>MSLFGTTSGFGTSGTSMFGSATTDNHNPMKDIEVTSSPDDSIGCLSFSPPTLPGNFLIAGSWANDVRCWEVQDSGQTIPKAQQMHTGPVLDVCWSDDGSKVFTASCDKTAKMWDLSSNQAIQIAQHDAPVKTIHWIKAPNYSCVMTGSWDKTLKFWDTRSSNPMMVLQLPERCYCADVIYPMAVVATAERGLIVYQLENQPSEFRRIESPLKHQHRCVAIFKDKQNKPTGFALGSIEGRVAIHYINPPNPAKDNFTFKCHRSNGTNTSAPQDIYAVNGIAFHPVHGTLATVGSDGRFSFWDKDARTKLKTSEQLDQPISAC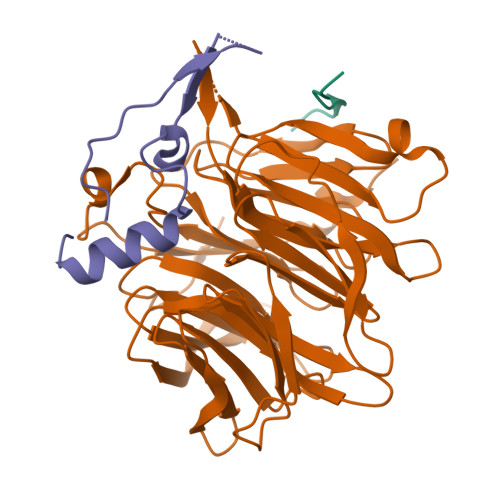CFNHNGNIFAYASSYDWSKGHEFYNPQKKNYIFLRNAAEELKPRNKK[2x];>MFNKSFGTPFGGGTGGFGTTSTFGQNTGFGTTSGGAFGTSAFGSSNNTGGLFGNSQTKPGGLFGTSSFSQPATSTSTGFGFGTSTGTANTLFGTASTGTSLFSSQNNAFAQNKPTGFGNFGTSTSSGGLFGTTNTTSNPFGSTSGSLFGPSSFTAAPTGTTIKFNPPTGTDTMVKAGVSTNISTKHQCITAMKEYESKSLEELRLEDYQANRKGPQNQVGAGTTTGLFGSSPATSSATGLFSSSTTNSGFAYGQNKTAFGTSTTGFGTNPGGLFGQQNQQTTSLFSKPFGQATTTQNTGFSFGNTSTIGQPSTNTMGLFGVTQASQPGGLFGTATNTSTGTAFGTGTGLFGQTNTGFGAVGSTLFGNNKLTTFGSSTTSAPSFGTTSGGLFGNKPTLTLGTNTNTSNFGFGTNTSGNSIFGSKPAPGTLGTGLGAGFGTALGAGQASLFGNNQPKIGGPLGTGAFGAPGFNTTTATLGFGAPQAPVALTDPNASAAQQAVLQQHINSLTYSPFGDSPLFRNPMSDPKKKEERLKPTNPAAQKALTTPTHYKLTPRPATRVRPKALQTTGTAKSHLFDGLDDDEPSLANGAFMPKKSIKKLVLKNLNNSNLFSPVNRDSENLASPSEYPENGERFSFLSKPVDENHQQDGDEDSLVSHFYTNPIAKPIPQTPESAGNKHSNSNSVDDTIVALNMRAALRNGLEGSSEETSFHDESLQDDREEIENNSYHMHPAGIILTKVGYYTIPSMDDLAKITNEKGECIVSDFTIGRKGYGSIYFEGDVNLTNLNLDDIVHIRRKEVVVYLDDNQKPPVGEGLNRKAEVTLDGVWPTDKTSRCLIKSPDRLADINYEGRLEAVSRKQGAQFKEYRPETGSWVFKVSHFSKYGLQDSDEEEEEHPSKTSTKKLKTAPLPPASQTTPLQMALNGKPAPPPQSQSPEVEQLGRVVELDSDMVDITQEPVLDTMLEESMPEDQEPVSASTHIASSLGINPHVLQIMKASLLTDEEDVDMALDQRFSRLPSKADTSQEICSPRLPISASHSSKTRSLVGGLLQSKFTSGAFLSPSVSVQECRTPRAASLMNIPSTSSWSVPPPLTSVFTMPSPAPEVPLKTVGTRRQLGLVPREKSVTYGKGKLLMDMALFMGRSFRVGWGPNWTLANSGEQLNGSHELENHQIADSMEFGFLPNPVAVKPLTESPFKVHLEKLSLRQRKPDEDMKLYQTPLELKLKHSTVHVDELCPLIVPNLGVAVIHDYADWVKEASGDLPEAQIVKHWSLTWTLCEALWGHLKELDSQLNEPREYIQILERRRAFSRWLSCTATPQIEEEVSLTQKNSPVEAVFSYLTGKRISEACSLAQQSGDHRLALLLSQFVGSQSVRELLTMQLVDWHQLQADSFIQDERLRIFALLAGKPVWQLSEKKQINVCSQLDWKRSLAIHLWYLLPPTASISRALSMYEEAFQNTSDSDRYACSPLPSYLEGSGCVIAEEQNSQTPLRDVCFHLLKLYSDRHYDLNQLLEPRSITADPLDYRLSWHLWEVLRALNYTHLSAQCEGVLQASYAGQLESEGLWEWAIFVLLHIDNSGIREKAVRELLTRHCQLLETPESWAKETFLTQKLRVPAKWIHEAKAVRAHMESDKHLEALCLFKAEHWNRCHKLIIRHLASDAIINENYDYLKGFLEDLAPPERSSLIQDWETSGLVYLDYIRVIEMLRHIQQVDCSGNDLEQLHIKVTSLCSRIEQIQCYSAKDRLAQSDMAKRVANLLRVVLSLHHPPDRTSDSTPDPQRVPLRLLAPHIGRLPMPEDYAMDELRSLTQSYLRELAVGSL[2x];>[2x]MFHLVDFQVTIAEILIIIMRTFRIAIWNLDVIISSIVRQLFKPLTKKNYSELDDEEPMELDYP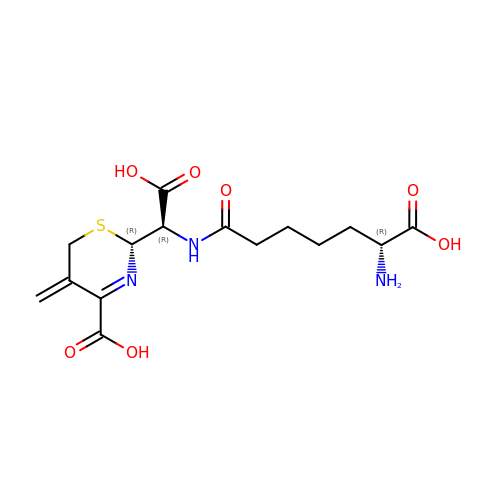CEPHALOSPORIN | C15 H21 N3 O7 S | JGKXEMYIHDYWCZ-JFUSQASVSA-N>AMNSLFASTARGLEELLKTELENLGAVECQVVQGGVHFKGDTRLVYQSLMWSRLASRIMLPLGECKVYSDLDLYLGVQAINWTEMFNPGATFAVHFSGLNDTIRNSQYGAMKVKDAIVDAFTRKNLPRPNVDRDAPDIRVNVWLHKETASIALDLSGDGLHLRGYRDRAGIAPIKETLAAAIVMRSGWQPGTPLLDPMCGSGTLLIEAAMLATDRAPGLHRGRWGFSGWAQHDEAIWQEVKAEAQTRARKGLAEYSSHFYGSDSDARVIQRARTNARLAGIGELITFEVKDVAQLTNPLPKGPYGTVLSNPPYGERLDSEPALIALHSLLGRIMKNQFGGWNLSLFSASPDLLSCLQLRADKQYKAKNGPLDCVQKNYHVAESTPDSKPAMVAEDYTNRLRKNLKKFEKWARQEGIECYRLYDADLPEYNVAVDRYADWVVVQEYAPPKTIDAHKARQRLFDIIAATISVLGIAPNKLVLKTRERQKGKNQYQKLGEKGEFLEVTEYNAHLWVNLTDYLDTGLFLDHRIARRMLGQMSKGKDFLNLFSYTGSATVHAGLGGARSTTTVDMSRTYLEWAERNLRLNGLTGRAHRLIQADCLAWLRE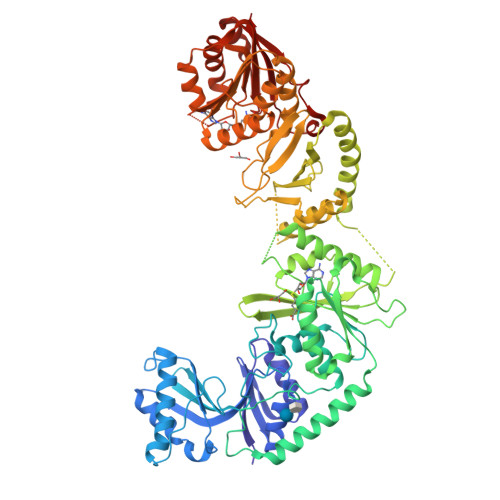ANEQFDLIFIDPPTFSNSKRMEDAFDVQRDHLALMKDLKRLLRAGGTIMFSNNKRGFRMDLDGLAKLGLKAQEITQKTLSQDFARNRQIHNCWLITAA[2x]> MSDSTPKTPRGFVVHTAPVGLADDGRDDFTVLASTAPATVSAVFTRSRFAGPS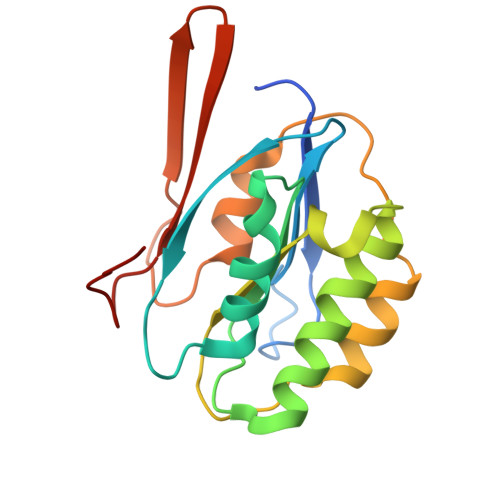VVLCREAVADGQARGVVVLARNANVATGLEGEENAREVREAVARALGLPEGEMLIASTGVIGRQYPMESIREHLKTLEWPAGEGGFDRAARAIMTTDTRPKEVRVSVGGATLVGIAKGVGMLEPDMA>[2x]MARKTKEDTQATREGILDAAEACFHEHGVARTTLEMIGARAGYTRGAVYWHFKNKSEVLAAIVERVHLPFMQELERTSTDQRDTPVHDLRAVMIHSFIELSEDERLRKTMEIMLRSDASANTRVLTEMQQAGFRDALDRMERALRRARDLGQLREGADPKIAARMLHATVLGVLHGAMVEPELMDLKRDGMLALDMTLAAYVKDGVFVPGTVPEPLPEA

The expression of SmeDEF is regulated by SmeT, a transcriptional repressor encoded upstream of smeDEF in the complementary DNA strand. SmeT belongs to the TetR family of transcriptional repressors. The members of this family show a characteristic helix-turn-helix DNA-binding motif at their N-terminal end and a C-terminal region involved in both dimerization and effector binding. The binding of SmeT to its operator region simultaneously represses smeDEF and smeT transcription by the steric interference of RNA polymerase binding to DNA.

The structure of the SmeT-triclosan complex involves one homodimer in the asymmetric unit, as seen for other TetR family members. A closer inspection of the electron density maps in the C-terminal domain showed a clear density in one of the subunits (A). This density was readily interpretable and allows the unambiguous placement of two molecules of the biocide (in agreement with the stoichiometry determined by fluorescence measurements) and the subsequent refinement. One of the triclosan (TCL1) molecules binds to the bottom of the ligand binding site, in close contact with helices α6, α7 and α8. The phenolic hydroxyl group forms a strong hydrogen bond with the Nδ atom of His167 (placed at 2.2 Å), anchoring this molecule almost parallel to helix α8. The hydroxyl group of the phenolic ring of TCL2 forms an H-bond with the Nδ atom of His67 (2.3 Å). The 2,4-dichlorophenoxy ring of TCL2 stacks against the phenol ring of Phe70 (3.4 Å). Residues 10–12, 21–34 and 45–55 that appeared disordered in apo SmeT become well ordered upon triclosan binding. However, no equivalent dense area was seen in subunit B. The volume of the triangle-shaped ligand binding cavity is 1030 Å3, which represents a notable increase with respect to the volume calculated for the apo SmeT structure (630 Å3), but similar to the calculated values for other TetR proteins. Due to the stabilization of the SmeT structure, the distance between the α-3 recognition helices of both subunits could be measured in the SmeT-triclosan complex, with 44.6 Å between the C-alpha atoms of Tyr49 (the N terminal of subunit B in the apo SmeT structure had to be modeled in order to estimate this length). This value is 10 Å longer than the distance between the B-form DNA major grooves, where these helices should bind.>MSVGTFSLPALPYAYDALEPSISAQIMELHHSKHHQTYVTNLNNALKTYSTALAANDVPSQIALQAAIKFNGGGHINHSLFWENLCPASSPDADPASAPELTA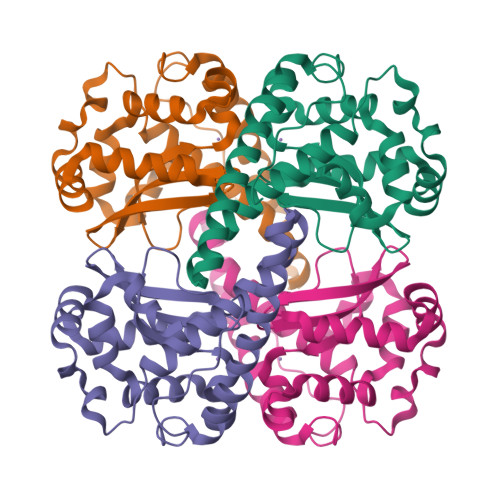EIAKTWGSLDKFKEAMGKALLGIQGSGWGWLVKEGSGLRIVTTKDQDPVVGGEVPVFGIDMWEHAYYLQYLNGKAAYVDNIWKVINWKTAEQRFKGDREDAFKILKASL[24x]Many streptococci adhere to protein-attached carbohydrates expressed on cell surfaces using Siglec-like binding regions (SLBRs). Siglec-like binding regions (SLBRs) are among the streptococcal adhesive modules that bind sialoglycans. SLBRs contain two adjacent modules: a Siglec domain, which shares some features with mammalian Siglecs, and a Unique domain13 with no close homologs outside of the family. The conserved sialic acid-recognition motif governs general specificity while sequence diversity in surrounding loop regions allows the SLBR to select between related sialoglycans.

To understand selectivity of these SLBRs for human glycans, we chose comparators from each branch for detailed study. From the first branch of the tree (blue in Fig. 2), we selected the SLBRs of the Hsa adhesin from S. gordonii strain Challis (termed SLBRHsa) and the equivalent SLBRs from Streptococcus sanguinis strain SK678 (SLBRSK678) and Streptococcus gordonii strain UB10712 (SLBRUB10712; see footnote). Although these three SLBRs are >80% identical in amino acid sequence, when they were tested with arrays containing 49 sialoglycans, they exhibited distinct binding profiles. In comparison, SLBRUB10712 and SLBRSK678 were more narrowly selective, although both bound to multiple sialoglycan ligands. Specifically, SLBRUB10712 bound strongly to 3’-sialyl-N-acetyllactosamine (3’sLn; Neu5Acα2-3Galβ1-4GlcNAcβ, Fig. 1b) and a small range of related structures, while SLBRSK678 bound to only two of the glycans on this array, 3’sLn and 6-O-sulfo-sialyl Lewis X (6S-sLeX; Neu5Acα2-3Galβ1-4(Fucα1-3)GlcNAc6Sβ, Fig. 1c). To reveal how similar SLBRs could include or exclude different sialoglycans, we determined crystal structures of these five SLBRs at resolutions between 1.0 Å and 1.7 Å. We then evaluated selectivity conferred by the FG loop where crystallographic analysis would suggest that the β-branching of SLBRHsaD356 excludes C3 fucosylation, while the larger, unbranched Gln of SLBRUB10712 and SLBRSK678 can bind fucosylated ligands. All three of these variants exhibited a substantial increase in binding for 6S-sLeX.

>GPGSDVANAVDTEAPQVKTGDYVVYRGESFEFYAEITDNSGQVNDVVVRNVELDKKTSQPYLTPGFIKFSTDNLGLPGNATVQNPLRTKIFGTVPLNEGIGYYTRYVVPTDSNGNTTRMVQNDNRNGLERFIITIKTQNEKYNPADPAITYVNQLSNLSQAERDAVAAAVRTANPQIPAAARITVSANGTVTITYPDSSTDTIPADRVVKDLAS[2x]> MTISRVKLLDTMVDTFLQKLVAAGSYQRFTDCYKCFYQLQPAMTQQIYDKFIAQLQTSIREEISDIKEEGNLEAVLNALDKIVEEGKVRKEPAWRPSGIPEKDLHSVMAPYFLQQRDTLRRHVQKQEAENQQLADAVLAGRRQVEE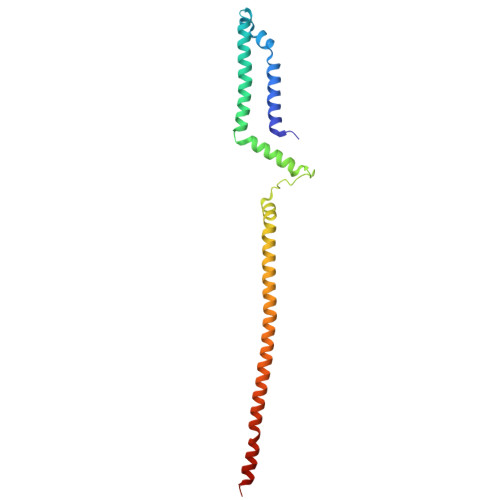LQLQVQAQQQAWQALHREQRELVAVLREPE1-(1H-indazol-5-yl)-3-(2-phenylethyl)urea 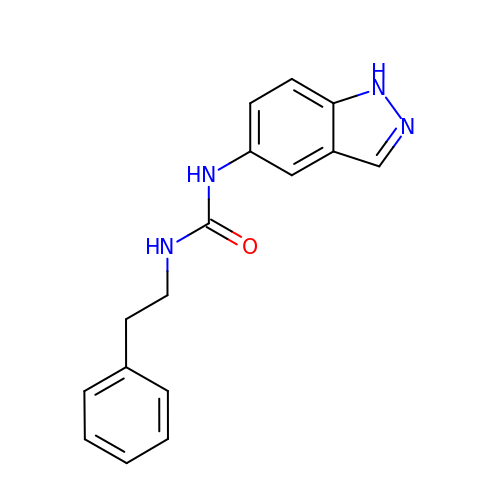| C16 H16 N4 O | XEZOXLSEWZHMQY-UHFFFAOYSA-N The replication-associated AP site repair protein HMCES protects cells from strand breaks, inhibits mutagenic translesion synthesis, and participates in repair of interstrand DNA cross-links derived from AP sites by forming a stable thiazolidine DNA–protein cross-link (DPC) to AP sites in single-stranded DNA (ssDNA). HMCES contains a catalytic SRAP (SOS Response Associated Peptidase) domain that is conserved across all domains of life. HMCES SRAP is similar in both sequence (29% identity/43% similarity) and structure to Escherichia coli (E. coli) YedK, with the highest degree of conservation within the DNA-binding channel and at the active site. An invariant cysteine at amino acid position 2 (Cys2) constitutes the extreme N-terminus after aminopeptidase removal of Met1 (18, 33) and is required for DPC formation in vivo and in vitro.

SRAP DPC formation likely proceeds through a Schiff base intermediate formed by nucleophilic attack of C1′ of the AP site by the α-amino group of Cys2 (22, 34, 42, 44). In the absence of the Cys2 thiolate side chain, SRAP does not form DPCs and instead generates DNA cleavage products indicative of DNA lyase activity. To visualize this Schiff base intermediate, we determined a 1.8-Å crystal structure of YedK C2A with AP-DNA in the presence of borohydride. The electron density shows a linear linkage consistent with a reduced imine between the N-terminal alanine and the ring-opened AP site. The active site residues in the trapped Schiff base structure are positioned almost identically to those in the wildtype YedK DPC. The main notable difference in the C2A DPC structure is that Glu105 only exhibits one conformer; the interaction between carboxylate and DNA phosphate is not observed. Interestingly, we did not observe a Glu105 conformer in contact with the DNA phosphate in the C2A DPC structure. This is consistent with our proposed mechanism in which Glu105 likely deprotonates the Cys2 sulfhydryl for thiazolidine ring closure in the last step of the reaction. Our YedK C2A crystal structure under reducing conditions confirms that the DPC reaction proceeds through a Schiff base intermediate and that the N-terminal amine is the initial cross-linking nucleophile.

>[2x]AGRFAQSQTREDYLALLAEDIERDIPYDPEPIGRYNVAPGTKVLLLSERDEHLHLDPVFWGYAPGWWDKPPLINARVETAATSRMFKPLWQHGRAICFADGWFEWKKEGDKKQPFFIYRADGQPIFMAAIGSTPFERGDEAEGFLIVTAAADQGLVDIHDRRPLVLSPEAAREWMRQEISGKEASEIAASGCVPANQFSWHPVSRAVGNVKNQGAELIQPVLEVLFQ> MERPAILPSGQILSNIEVHSHRALFDIFKRFRSDDNNLYGAEFDALLGTYCSTLSLVRFLELGLSVACVCTKFPELSYVAEGTIQFEVQQPMIARDGPHPADQPVHNYMIKRLDRRSLNAAFSIAVEALGLISGENLDGTHISSAMRLRAIQQLARNVQAVLDSFERGTADQMLRVLMEKAPPLSLLAPFTLYEGRLADRVACAALVSELKRRVRDDTFFLTKHERNKDAVLDRLSDLVNCTAPSVAVARMTHADTQGRPVDGVLVTTAGVRQRLLHHVLTLADTHADVPVTYGEMVIANTNLVTALVMGKAVSNMDDVARYLLGGEPAPDDGKPVGSARVRADLVVVGDRLVFLEALEKRVYQATQVPYPLVGNLDVTFVMPLGVFKPAADRYARHAGSFAPTPGLPDPRTHPPRAVHFFNKDGVPCHVTFEHAMGTLCHPSFLDVDATLAALRQEPAEVQCAFGAYVADARPDALVGLMQRFLEEWPGMMPVRPRWAAPAAADQLLAPGNADLRLELHPAFDFFVAPEVDVPGPFAVPQVMGQVRAMPRIINGNIPLALCPVDFRDARGFELSVDRHRLAPATVAAVRGAFRDANYPMVFYIIEAVIHGSERTFCALARLVAQCIQSYWRNTHNAAFVNNFYMVMYINTYLGNGELPEDCAAVYKDLLEHVHALRRLIGEFTLPGDPLGNQPQEELNHALADATLLPPLIWDCDPILYRDGLAERLPELRVNGAHFQHILWVEMAQVNFRNVGGGLVHNRPVRNENQPLHPHHDAEWSVLSKIYYYAVVPAFSRGNCCTMGVRYDRVYQLVQTMVVPETDEEVGTDDPRHPLHPRNL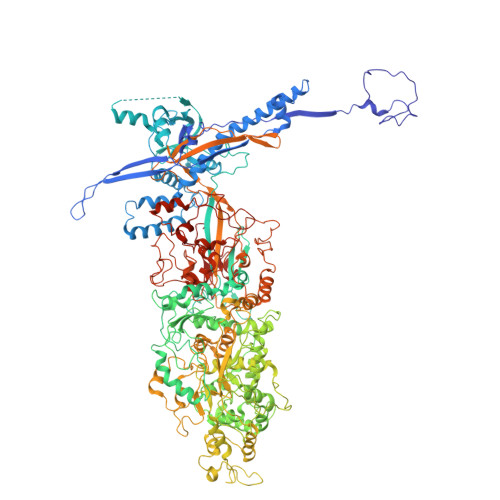VPNSLNVLFHNACVAVDADAMLILQETVTNMAERTTPLLASVAPDAGMATVATRDMRTHDGSLHHGLLMMAYQPNDATLLEGAFFYPAPVNALFACADHLGAMRDVGAEVRAAAQHVPCVPHFLGANYYATVRQPVAQHAAQSRADENTLSYALMAGYFKMSPVAFTHQLRRQLHPGFALTVVRQDRFATENVLFAEKASESYFMGQMQVARTESGGGLHLQLTQPRANVDLGVGFTAAYAAAALRAPVTDMGNLPQNLFATRGAPPMLDADADDYLRRTVNAGNRLAPVPVFGQMLPQVPAGLARGQQSVCEFIATPVSVDLAYFRRACNPRGRAAGEVHGEEGLMFDHSHADPAHPHRATANPWASQRHSYADRLYNGQYNMSGPAYSPCFKFFTPAEAVAKSRGLARLIADTGAAASPTSNGEYQFKRPVGAGELVEDPCALFQEAYPPLCASDSALLRTPLGAEEHFAQYLIRDESPLKGCFQHASA>GQKRSLSREALQKDLDDNLFGQHLAKKIILNAVFGFINNPKPKKPLTLSLHGWTGTGKNFVSKIIAENIYEGGLNSDYVHLFVATLHFP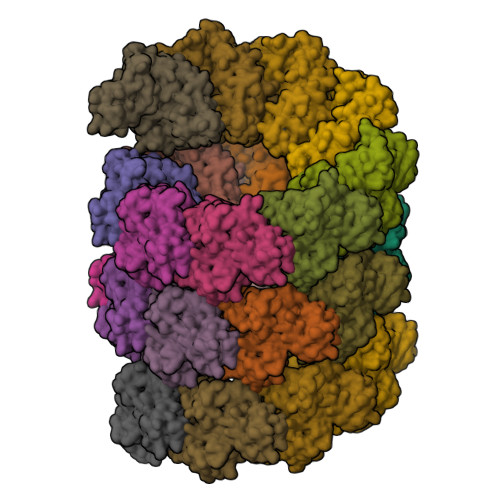HASNITLYKDQLQLWIRGNVSACARSIFIFDEMDKMHAGLIDAIKPFLDYYDLVDGVSYQKAMFIFLSNAGAERITDVALDFWRSGKQREDIKLKDIEHALSVSVFNNKNSGFWHSSLIDRNLIDYFVPFLPLEYKHLKMCIRVEMQSRGYEIDEDIVSRVAEEMTFFPKEERVFSDKGCKTVFTKLDYYYDD[25x]> MSFITAFIWAYFLWLVLTAGSKGMLWSTQELIAGLIFASIVGYSTRNIIGEKASRFLNPVKWILFVAYAPVLFWGMVKANLDVAYRVITGKIRPGIVRVPVELENDAQYTILSNSITLTPGTLTVEACPEEKALYVHWINIPEGLEWPENSEPVSGPFEKWARRLGA;> MIFFYATLLIGIAGIITFIRLALGPTVPDRVVAVDTLNTLIVAIMLLLGAAYERAIYIDIAIVYALLSYVGTLVIAKYLQGGLQ;> MIAYYLIIAFLGISVTFNMLGSIALHRFPDVYTRLHGATKCTTFGTIFAALAVITHAIVKLQATGNPKYLQMAIHSFVAMLALLLTNPVGAHAIAKAAHKTGYLPKRAVVDAYLEKERGEKNES;> MHISKKKGVRKMNLDMIIQFIVLGGIILSSVLMIVTRDLLVAVLASAAMSLLLSLEFYMLHAPDVAIAEAAVGAGVVTALVMYAISKTERWEREAP;> MKRALGFLSLLVIFASLLVALSPEYGIKFGVGGEDWLKYRYTDNYYIEHGIEEVGGTNIVTDIVFDYRGYDTLGEATVLFTAIAG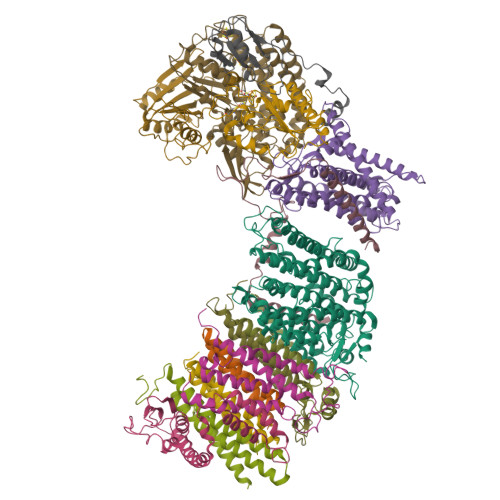AVALLRPWRREENE;> MNEDMGVIVRTNARALIPFIGIFGAYIVTHGHLTPGGGFQGGATIAGAGVLFLIAFGVKAAKEKINKNLYSALEGLGGLVFLGAAMLGLSVAFFYNILWHEGPIFNSSPGTLLSAGFLPIMNLGVGLKVFTGLVSALFALSVFRRWKS;> MIAFQYLTATIMILLGIYALLYKRNLIKLVLALNLIDSGIHLLLISEGYRMENGIPPTAPIYTGYEGGAMVAPIPQALVLTSIVIGVCVLSLAIALTVNAYRHYGTLDVTKLRRLRG;> MTWLPFIIIIPLLGAFSMPIVSLLKGKAKEIWASMISFATLIVGIQVFREVWSKGTIVYTLGAPNPFGKATFPIRIVWEVDKFGALMVLIVTFVSFLAVIYSIEYMKHDTGLEKFYTLILILELGMLGIAITGDIFNFYVFLEIMSIASYALVAFRNDTWEGIEAGIKYMFAGSLASSFVLLGIALLYGQYGTLTMGYLAVKIAENPTIVAKVALALFIGGLLFKSGAAPVHMWLADAHPAAPSSISAMLSGLVIKIGGIYAIARIVFSIFSPTINLGTIGWIIIIFACITLIVGNAMAVVQEDLKRLLAYSSVGQIGYILLGLGIGMVAYGTRVGEIALAGAIYHTVNHALMKALLFLVAGAVIHEIGTRNMNELSGLAKTMPKTTFAFLIGAAAIVGLPPLNGFASKWLIYESSALFNPILGAIAVIGTVFCTAAYVRALFTFFGRPSEKVTNARDPGIAMMLPMIILVVTIIVMGFFPWQISDRIMVPTARALWDVIDYISSLMGGG;> MFGYWDPLYFIIVFIIGLILAYLLNLWAKKSGMGTREVGEGTKIFISGEDPEKVIPGFEHLEGYYTGRNTMWGLVNGVKKFFATLKNDHTGLLPDYVSYLLMTTAFILVILLLRG;> MTNNSERKRLEKRIAQLCKFIGRSPWVFHVNSGSCNGCDIEIIAALTPRYDAERFGVKLVGSPRHADILLVTGPVTNQSLERVKLVYEQTPDPKIVIAIGACPTGGSVFYESPFTNAPLDRIIPVDVFVPGCPPRPEAILHGVVLALEKLAKMIKGEVPPEEGEENE;> MSKAEMVANKIKERFPNAEVVVKTNKWGRERVWVRISREEYKELMKFIRELDPEAHYSIGIEQDWGDELGFLNHILLFYDEPPGVSLLIDVHAPKDNPVLPDTSDIFPISLQFEREGMEMVGLDFEGAPDKRRLFLPDDFPEGIYPLRTDEKGVPEEMVKNAGHPYLLRREKK;> MKKVEYWVKIPFGPIHPGLEEPEKFIITLDGERIVNVDVKLGYNLRGVQWIGMRRNYVQIMYLAERMCGICSFSHNHTYVRAVEEMAGIEVPERAEYIRVIVGELERIHSHLLNLGVVGHDIGYDTVLHLTWLARERVMDVLEAVSGNRVNYSMVTIGGVRRDIGEKQKRLILDMIKYYREVLPQIEDVFLHDSTIEARLRDVAVVPKKLAIEMGAVGPTARGSGIKEDSRWSEQLGVYPDLGIKPVTPEDVTGEKARGDVYDRMAVRIGELWMSLDLLEHALDQMPEGKIKTFPKDNILVAKLKLLGDGEGIGRYEAPRGELVHYVRGQKGRDGPVRWKPREPTFPNLFTIAKALEGNELADLVVAIASIDPCLSCTDR;> MKIVYGVIGLILIYIYVSVVSLLFSGIDRKLVARMQRRIGPPILQPFYDFLKLMSKETIIPKTANFMFKAAPILMLATVIALLAYTPLGFPPIFGTKGDIIVFIYLLTLADFFLVVGVMSSGSPYGRIGAARGIALLVSREPAMMLGVFAVMWAISKLGVEKPFSLSSLYEHTIWDFGPVAWVAGVVLIYVFMAWLASEIEVGFFNIPEAEQEIAEGTLVEYSGRYLGIIKLAESIKEFIAASLVVAVLFPWQLNIPGVQGYLINLLLHTLKVFIVLLVSKTIFRTITGRLKISQAVNLLWTRVFTASVIGALLLALGVML;> MIRLPLLPTVIKNLFKKPATNPFPKTEPVPVPEDFRGKLVYNVDKCVGCRMCVTVCPAGVFVYLPEIRKVTLWIGRCVMCKQCVDVCPTAALQMSDEFLLASYDKYDAKLIYLTPEEAEDIKKKLEEANKAKAEKQASK> GMSEALSDSGLPPVQRVVTGHDAHGRAVFKSEDVTPTRMIPSGDASFLLVWTTATVPADNND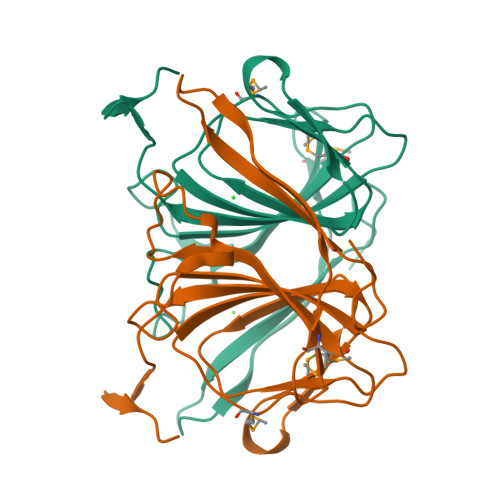ETDGRQREAGLTLDGGSVIRVVDMLPGKESPMHRTNSIDYGIVLEGEIELELDDGAKRTVRQGGIIVQRGTNHLWRNTTDKPCRIAFILIEAPAYLHNGQPLPEDKPDHK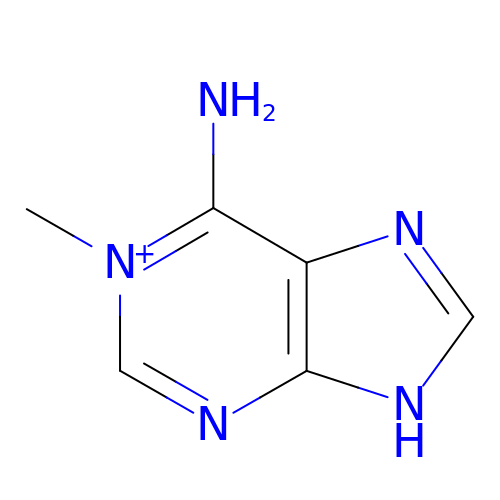6-AMINO-1-METHYLPURINE | C6 H8 N5 | DYGBIJOMQSXREB-UHFFFAOYSA-O> MSADSSPLVGSTPTGYGTLTIGTSIDPLSSSVSSVRLSGYCGSPWRVIGYHVVVWMMAGIPLLLFRWKPLWGVRLRLRPCNLAHAETLVIEIRDKEDSSWQLFTVQVQTEAIGEGSLEPSPQSQAEDGRSQAAVGAVPEGAWKDTAQLHKSEEAKRVLRYYLFQGQRYIWIETQQAFYQVSLLDHGRSCDDVHRSRHGLSLQDQMVRKAIYGPNVISIPVKSYPQLLVDEALNPYYGFQAFSIALWLADHYYWYALCIFLISSISICLSLYKTRKQSQTLRDMVKLSMRVCVCRPGGEEEWVDSSELVPGDCLVLPQEGGLMPCDAALVAGECMVNESSLTGESIPVLKTALPEGLGPYCAETHRRHTLFCGTLILQARAYVGPHVLAVVTRTGFCTAKGGLVSSILHPRPINFKFYKHSMKFVAALSVLALLGTIYSIFILYRNRVPLNEIVIRALDLVTVVVPPALPAAMTVCTLYAQSRLRRQGIFCIHPLRINLGGKLQLVCFNKTGTLTEDGLDVMGVVPLKGQAFLPLVPEPRRLPVGPLLRALATCHALSRLQDTPVGDPMDLKMVESTGWVLEEEPAADSAFGTQVLAVMRPPLWEPQLQAMEEPPVPVSVLHRFPFSSALQRMSVVVAWPGATQPEAYVKGSPELVAGLCNPETVPTDFAQMLQSYTAAGYRVVALASKPLPTVPSLEAAQQLTRDTVEGDLSLLGLLVMRNLLKPQTTPVIQALRRTRIRAVMVTGDNLQTAVTVARGCGMVAPQEHLIIVHATHPERGQPASLEFLPMESPTAVNGVKDPDQAASYTVEPDPRSRHLALSGPTFGIIVKHFPKLLPKVLVQGTVFARMAPEQKTELVCELQKLQYCVGMCGDGANDCGALKAADVGISLSQAEASVVSPFTSSMASIECVPMVIREGRCSLDTSFSVFKYMALYSLTQFISVLILYTINTNLGDLQFLAIDLVITTTVAVLMSRTGPALVLGRVRPPGALLSVPVLSSLLLQMVLVTGVQLGGYFLTLAQPWFVPLNRTVAAPDNLPNYENTVVFSLSSFQYLILAAAVSKGAPFRRPLYTNVPFLVALALLSSVLVGLVLVPGLLQG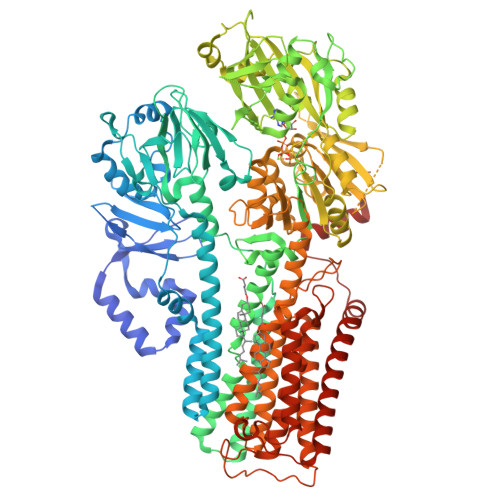PLALRNITDTGFKLLLLGLVTLNFVGAFMLESVLDQCLPACLRRLRPKRASKKRFKQLERELAEQPWPPLPAGPLR>[2x]SKTRQTFSWVGRPLPNRKQFQQMYREICMKIND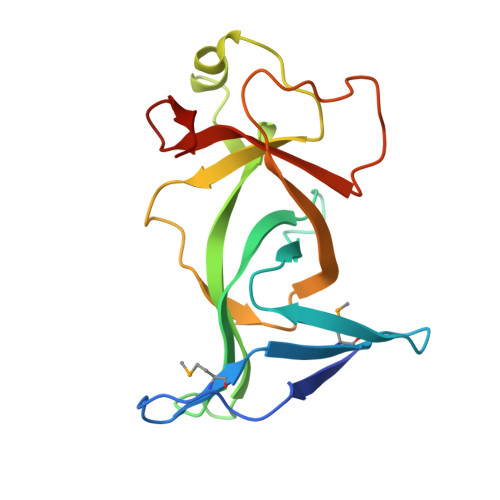GSEIHIKVGQFVLIQGEDNKKPYVAKLIELFQNGAEVPPKKCARVQWFVRFLEIPVSKRHLLGRSPPAQEIFWYDCSDWDNKINVETIIGPVQVVALAPEEVIPVDQKSEETLFVKLSWNKKDFAPLPPE> MRRCGNDRAVALLRATTEAMRLVKLKLSPDRTRNEEIQDRQNAFVWSDEHIFRPHQHFTHDPCSWSRSLEQSMKKQRKLSMVERLRSLEQRQLEEKQSASATAGGSSKCANHMDGEKAEGPRFYGAVGDSEDLKEYVANEDYFYTMQQEEKPNDPPLQELVDEVQSLHVLLSSPRYEDTPLATVERLQCAYSEALRCVFDRVRNASVGKTMSCNALLFSWSLLLQGVPALLESLAEKRTEECLVRALSTVHEALNIVLQEFNRITHSKERVELLPLEGWIESLDVVTHPLTNKDYTSLKG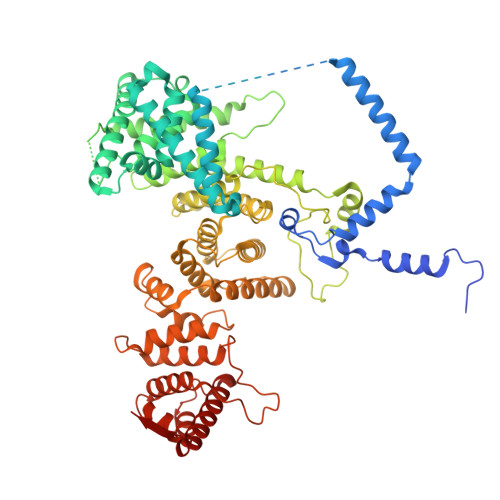NIRLPESSFKPQCKLDSATVEFVHSRAIQAAAIRMIENDQSDVETEPLDPYHLYILLRCMVRLAEKGVNDSHIHRAALLTGMVGERIFSSLERTVAPPRRYSLRHALLGKQLRDASKPHAIPLDVCAPPGGVKKPPTAADDVLLLTRACTLLMKVATNVLPQTKFKVLETVDTVLKTLSYAPNYDLSTADTVIFSNMVLEELHHVDEASATDRHLRVLLLLSRLRLSMCADRSALSHLFSCLCNLLPPHSIQQDKLREWKRLRGLVMRHLLYSVRGEEVEQHYTRVLKSSETWVEHLAFGQYSGGLPLSLWLEACHIYLTAGRKLTVSCAEALITLRGRCKDGGVLRSSNSAGVGPLDFVSVTLLAQLLEVVSHGCCSADDLVASPVAWDKVRQTIQGAIGEDENTIQLLRAGRLCVADRQATGSLVTTYP> GSHMASMKKKGSVVIVGRINLSGDTAYAQQTRGEEGCQETSQTGRDKNQVEGEVQIVSTATQTFLATSINGVLWTVHHGAGTRTI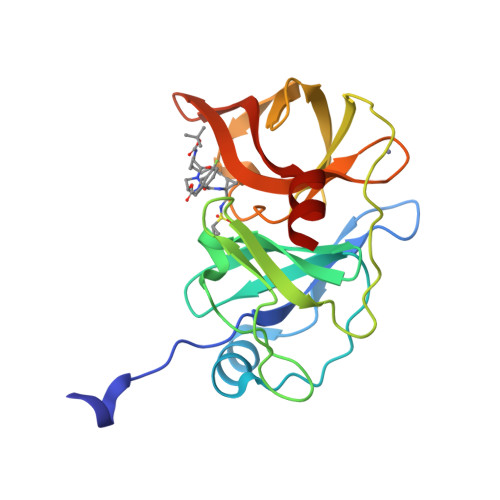ASPKGPVTQMYTNVDKDLVGWQAPQGSRSLTPCTCGSSDLYLVTRHADVIPVRRRGDSRGSLLSPRPISYLKGSSGGPLLCPAGHAVGIFRAAVSTRGVAKAVAFIPVESLETTMRSP>PIMLRGGRQEYEPVGPGLIAAWLKQVQEHGLTHPATITYFGVISINFTSVDINMLLNVTPGFAAEKQLVIDKIKEKAIAWDEMHPPPPADAAGPVPLTSDQIRGIGLSPEEAAGPRFADARTLYRTWVLEALQECQRTISPLE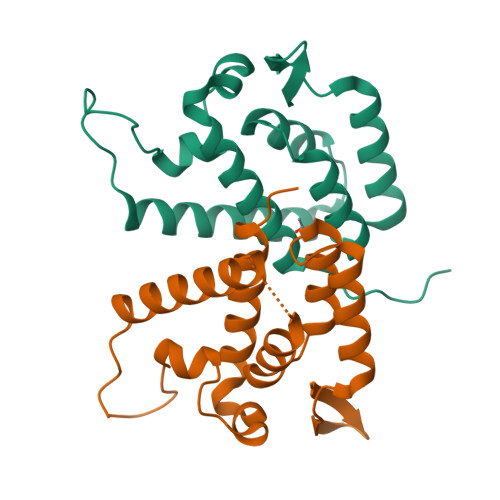HHHHHH[2x]> MGKYNLILSEYLSFIYNSQSAVQIPIYYSSNSELENRCIEFHSKCLENSKNGLSLKKLFVEYSDVIENATLLSILSYSYDKYNAVERKLVKYAKGKPLEADLTVNELDYENNKITSELFPTAEEYTDLLMDPAILTSLSSNLNAVMFWLEKHENDVAEKLKIYKRRLDLFTIVASTVNKYGVPRHNAKYRYEYEVMKDKPYYLVTWANSSIEMLMSVFSHEDYLIARELIVLSYSNRSTLAKLVSSPMSILVALVDINGTFITNEELELEFSNKYVRAIVPDQTFDELKQMLDNMRKAGLTDIPKMIQDWLVDCSIEKFPLMAKIYSWSFHVGFRKQKMLDAALDQLKTEYTEDVDDEMYREYTMLIRDEVVKMLEEPVKHDDHLLQDSELAGLLSMSSASNGESRQLKFGRKTIFSTKKNMHVMDDMANGRYTPGIIPPVNVDKPIPLGRRDVPGRRTRIIFILPYEYFIAQHAVVEKMLIYAKHTREYAEFYSQSNQLLSYGDVTRFLSNNSMVLYTDVSQWDSSQHNTQPFRKGIIMGLDMLANMTNDARVIQTLNLYKQTQINLMDSYVQIPDGNVIKKIQYGAVASGEKQTKAANSIANLALIKTVLSRISNKYSFATKIIRVDGDDNYAVLQFNTEVTKQMVQDVSNDVRETYARMNTKVKALVSTVGIEIAKRYIAGGKIFFRAGINLLNNEKKGQSTQWDQAAVLYSNYIVNRLRGFETDREFILTKIMQMTSVAITGSLRLFPSERVLTTNSTFKVFDSEDFIIEYGTTDDEVYIQRAFMSLSS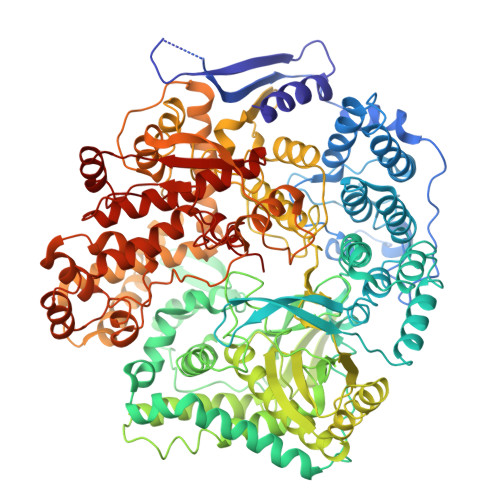QKSGIADEIAASSTFKNYVSRLSEQLLFSKNNIVSRGIALTEKAKLNSYAPISLEKRRAQISALLTMLQKPVTFKSSKITINDILRDIKPFFTVNEAHLPIQYQKFMPTLPDNVQYIIQCIGSRTYQIEDDGSKSAISRLISKYSVYKPSIEELYKVISLHENEIQLYLISLGIPKIDADTYVGSKIYSQDKYRILESYVYNLLSINYGCYQLFDFNSPDLEKLIRIPFKGKIPAVTFILHLYAKLEVINHAIKNGSWISLFCNYPKSEMIKLWKKMWNITSLRSPYTNANFFQD>MQATLIKPTIFTHQPILEKLFKSQSMTQEESHQLFAAIVRGELEDSQLAAALISMKMRGERPEEIAGAASALLADAQPFPRPDYDFADIVGTGGDGTNSINISTASAFVAASCGAKVAKHGNRSVCQPLAGSCDLLQAFGI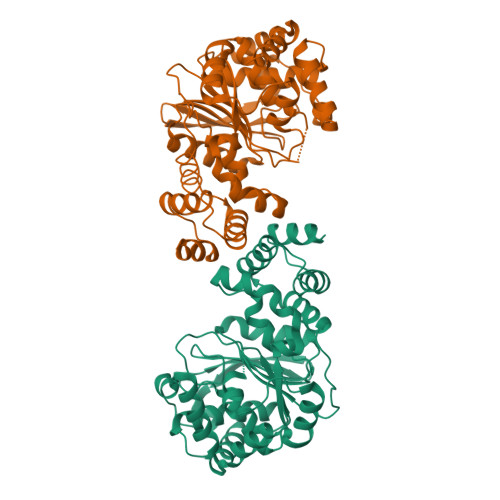RLDMSAEDSRQALDDLNVCFLFAPQYHTGFRHAMPVRQQLKTRTIFNVLGPLINPARPPKALIGVYSPELVLPIAQALKVLGYKNAAVVHGGGMDEVAIHTPTQVAELNNGEIESYQLSPQDFGLQSYSLNALQGGTPEENRDILARLLQGKGDAAHARQVAANVALLLKLFGQDNLRHNAQLALETIRSGTAFERVTALAARG[4x]> APVTSPAWADDPPATVYRYDSRPPEDVFQNGFTAWGNNDNVLEHLTGRSCQVGSSNSAFVSTSSSRRYTEVYLEHRMQEAVEAERAGRGTGHFIGYIYEVRADNNFYGAASSYFEYVDTYGDNAGRILAGALATYQSEYLAHRRIPPENIRRVTRVYHNGITGETTTTEYSNAR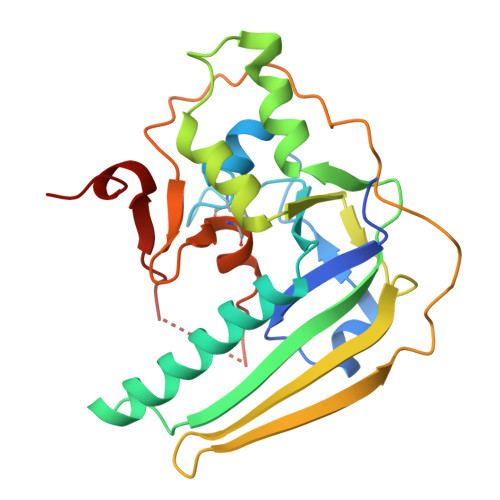YVSQQTRANPNPYTSRRSVASIVGTLVRMAPVVGACMARQAESSEAMAAWSERAGEAMVLVYYESIAYSF>EPKLDMNKQKISPAEVAKHNKPDDCWVVINGYVYDLTRFLPNHPGGQDVIKFNAGKDVTAIFEPLHAPNVIDKYIAPEKKLGPLQGSMPPELVCPPYAPGETKEDIARKEQLKSLLPPLDNIINLYDFEYLASQTLTKQAWAYYSSGANDEVTHRENHNAYHRIFFKPKILVDVRKVDISTDMLGSHVDVPFYVSATALCKLGNPLEGEKDVARGCGQGVTKVPQMISTLASCSPEEIIEAAPSDKQIQWYQLYVNSDRKITDDLVKNVEKLGVKALFVTVDAPSLGQREKDMKLKFSNTKAGPKAMKKTNVEESQGASRALSKFIDPSLTWKDIEELKKKTKLPIVIKGVQRTEDVIKAAEIGVSGVVLSNHGGRQLDFSRAPIEVLAETMPILEQRNLKDKLEVFVDGGVRRGTDVLKALCLGAKGVGLGRPFLYANSCYGRNGVEKAIEILRDEIEMSMRLLGVTSIAELKPDLLDLSTLKARTVGV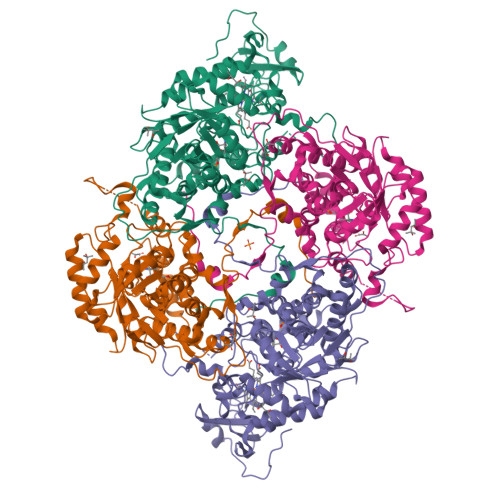PNDVLYNEVYEGPTLTEFEDA[2x]> NNVGPIIRAGDLVEPVIETAEIDNPGKEITV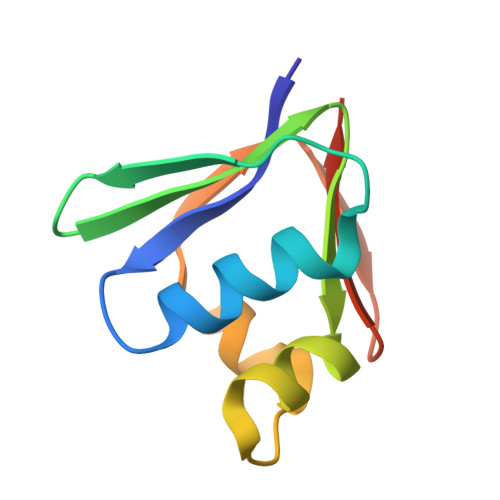EDRRAYVRIAAEGELILTRKTLEEQLGRPFNMQELEINLASFAGQIQADEDQIRFYFDKTM>MGRVLIIGAGGVGTVVAHKVAQNADVFTDIMIASRTKSKCDDIVKAIGNPNIKTAQVDADNVDELVALFNDFKPEMVINVALPYQDLTIMEACLKAEVNYLDTANYEPKDEAHFEYSWQWAYHERFKEAGLTAILGCGFDPGVSGIYTAYAAKHYFDEIQYLDIVDCNAGNHHKAFATNFNPEINIREITQNGRYYENGQWVTTGPLEIHKDLTYPNIGPRDSYLLYHEELESLVKNFPTIKRARFWMTFGQEYLTHLRVIQNIGMARIDEIDYNGQKIVPLQFLKAVLPNPQDLGENYEGETSIGCRIRGLKDGKERTYYVYNNCSHEEAYKETGMQGVSYTTGVPAMIGAMMFFKGEWKRPGVNNVEEFNPDPFMEQLNKQGLPWHEVFDGNLEL[2x]

The polyamine biosynthetic pathway used by most gut microbes differs from that used by human cells. This alternative pathway employs carboxyspermidine dehydrogenase (CASDH), an enzyme with limited characterization. Carboxyspermidine dehydrogenase, from two major gut microbes, performs the reductive condensation of aspartate semi-aldehyde (ASA) and putrescine using NADPH as a coenzyme, in the formation of carboxyspermidine. CASDH is a homolog of enzymes that perform similar chemistry including saccharopine dehydrogenase, L-lysine 6-dehydrogenase, and homospermidine synthase. In this study, we investigated the largely uncharacterized carboxyspermidine dehydrogenase that produces carboxyspermidine as a precursor to the polyamine spermidine in an alternative polyamine biosynthetic pathway first identified in Vibrio alginolyticus. This alternate pathway is known to be present in many bacterial species including a majority of the most prevalent human gut microbes.

The solution of a 1.94 Å BfCASDH X-ray crystal structure, with NADP+ bound, allowed a characterization of CASDH domain structure and active site arrangement, as well as a comparison with homolog enzymes from the saccharopine dehydrogenase, L-lysine 6-dehydrogenase, and homospermidine synthase families. BfCASDH is composed of three domains. An NAD(P)-binding domain spans residues 1 to 136 and is a canonical Rossmann-fold domain with 321456 β-strand topology encoding a GXGXXG loop, from residues 8 to 13, that stabilizes the diphosphate backbone of NADP+. The catalytic domain, from residue 137 to 250 and 290 to 397 is an α/ β domain composed of ten β-strands, six α-helices, and one 3/10 helix. A dimerization domain interrupts the catalytic domain from residue 251 to 289 and is composed of two α helices and two β strands that form a small antiparallel sheet. The descriptions below refer to chain B but include the slight differences observed in chain A. The hydrogen bonding network surrounding the C2′-phosphate of the 5′-phosphate adenosine-2′,5′-bisphosphate moiety suggests a basis for NADP selectivity for BfCASDH. The guanidino group of Arg45 hydrogen bonds with two of the phosphoryl oxygens. NADP+ is positioned in a V-shaped active site with two entrance channels, one through the NAD(P)-binding domain and the other through the catalytic domain and flanked by α 9 of the dimerization domain. His228 is positioned to serve as a general base in the catalytic cycle. The proximity of the dimerization domain, and our observation of cooperative enzyme kinetics, suggests communication with structural elements of the catalytic domain that overlay the active site and across the dimeric interface.>GSHMASAKAATKLADGKYNIAFTVWKGDKDESSRMNRYFESPATLTVKNGKQYVSFKVKDSTSIKSFQVEKD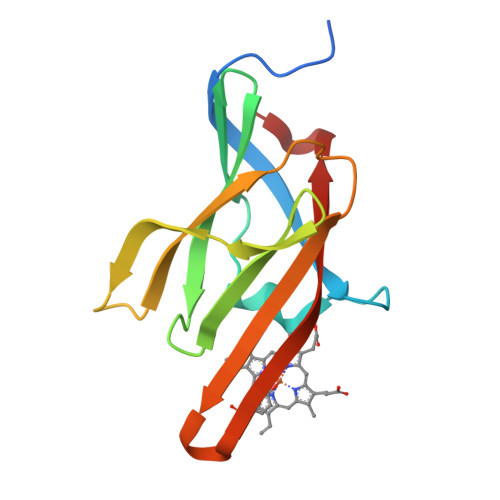GQFVETTVLSENKKDNTRVVEFEVADLSKKLNGKVKINIPIINYNASYDIRFVFDGNSIK[2x]FXII circulates in the blood as an 80-kDa single-chain polypeptide zymogen with no detectable enzymatic activity. The FXII Arg353–Val354 peptide bond is cleaved by kallikrein, generating α-FXIIa, which has a heavy chain of 50 kDa, connected to a light chain of 28 kDa by the Cys340–Cys467 disulfide bridge. Subsequent cleavage of α-FXIIa results in loss of the heavy chain and generation of the isolated protease domain termed β-FXIIa, which contains only a nine amino acid peptide heavy chain remnant disulfide bonded to the protease domain. Here, we describe the first crystal structures of the FXII protease domain, which reveals a zymogen-like conformation.

FXIIc is a protein-engineered zymogen-like construct with two additional residues present at the N-terminus, resulting from the cloning strategy, that effectively block the native N-terminal residue Val354. We term this the zymogen-like construct, as it is similar to the result of protein engineering of the N-terminus of FXa to induce zymogenicity. FXIIc crystallized more readily than FXIIac under a range of conditions for both glycosylated and deglycosylated samples at 19 °C. Data were collected to 2.1-Å resolution for the deglycosylated FXIIc sample, and Fig.2D shows the electron density in the region of the active site residue Ser195. In a second crystal form of the deglycosylated light chain, the S1 pocket loops are ordered, and a short α-helix in the 180-loop of the structure results in an enlarged and distorted S1 pocket with a buried conformation of Asp189, which is critical for P1 Arg substrate recognition. In FXIIc, Arg73 extends its side chain guanidinium group from the 70-loop of the N-terminal β-barrel to form a direct salt bridge with the buried Asp194 side chain. The Arg73 side chain from the 70-loop is stabilized by a number of interactions with the 140-loop, resulting in encirclement of the Arg73 guanidinium group and the formation of hydrogen bonds via the side chain of Gln151. In HGFA, the 140-loop forms a hairpin-like structure folded up against the side of the C-terminal β-barrel, interacting with the 180-loop close to the entrance of the S1 pocket. This folded-up 140-loop conformation is commonly observed in activated proteases, and contrasts with FXIIc, in which the 140-loop extends away from the body of the C-terminal β-barrel. All residues that contact the inhibitor in HGFA are in different positions in FXIIc, by virtue of the concerted coiling of residues 189–194 into the FXII S1 α-helix. In the current study, we report the first crystal structures of the FXII protease domain light chain. Both FXIIac and protein-engineered zymogen-like construct FXIIc structures reveal the conformational hallmarks of a zymogen, owing to the lack of an oxyanion hole, a disordered (FXIIac) or helical (FXIIc) 180-loop, and an extended 140-loop.

> RSVVGGLVALRGAHPYIAALYWGHSFCAGSLIAPCWVLTAAHCLQDRPAPEDLTVVLGQERRNHSCEPCQTLAVRSYRLHEAFSPVSYQHDLALLRLQEDADGSCALLSPYVQPVSLPSGAARPSETTLCQVAGWGHQFEGAEEYASFLQEAQVPFLSLERCSAPDVHGSSILPGMLCAGFLEGGTDACQGDSGGPLVCEDQAAERRLTLQGIISWGSGCGDRNKPGVYTDVAYYLAWIREHTVSHHTGTRHHHHHH>[2x]EVQDVNDSSWKEFVLESEVPVMVDFWAPWCGPCKLIAPVIDELAK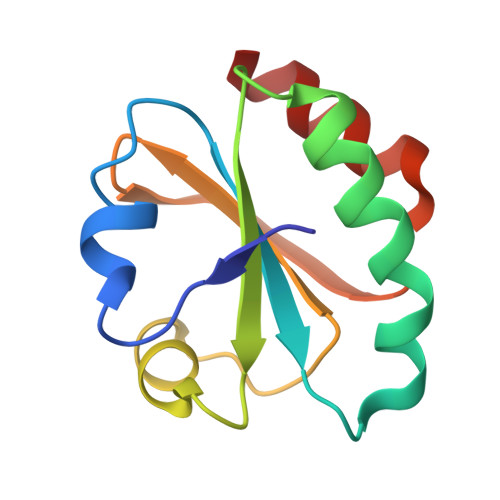EYSGKIAVYKLNTDEAPGIATQYNIRSIPTVLFFKNGERKESIIGAVPKSTLTDSIEKYL>GARQVFDDKLLAVISGNSIGVLATIKHDGRPQLSNVQYHFDPRKLLIQVSIA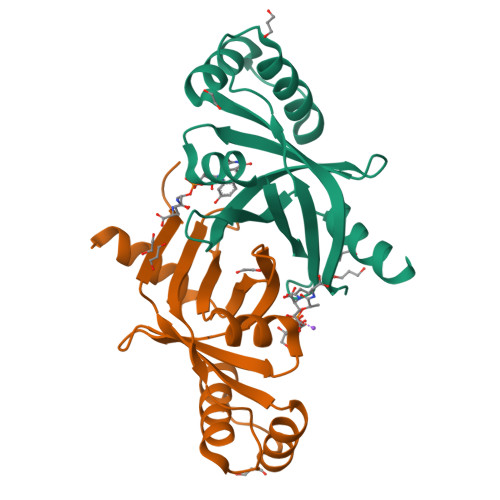EPRAKTRNLRRDPRASILVDADDGWSYAVAEGTAQLTPPAAAPDDDTVEALIALYRNIAGEHSDWDDYRQAMVTDRRVLLTLPISHVYGLPPGMR[2x]>[4x]GSTQIDKPAVVSLPSSEQFY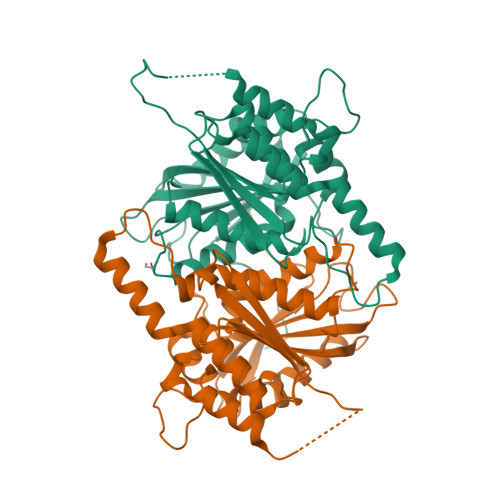LNNSRGERYLIQVSWPLHWKDHKPDTDRNDVPLIYIVDGNALFLTATEALWRRSADSHYCGGGIVVAIGYPLEGTGKVYHRVRRGFDLTVPTPDSPVEGHGGADILLDFIAETVRPAVRERFPDVSVSREALYGHSYGGLFALHALFTRPSMFDAYIASSPSIWWNGRCILNEAKAFTRKIKENGAYTNGEKKLPSLMMYLGGLEQDPRRWNDEPDESWEGRKRDAEAFNMKVNLLELMGLIRGCTRLHAVSFSEYAGEDHGTVMACSLGRGFSTFMEDWPVPREESV>[2x]PRERPHTSGHHGAGEARATAPSTVSPYGPEARAELSSRLTTLRNTLAPATNDPRYLQACGGEKLNRFRDIQCRRQTAVRADLNANYIQVGNTRTIACQYPLQSQLESHFRMLAENRTPVLAVLASSSEIANQRFGMPDYFRQSGTYGSI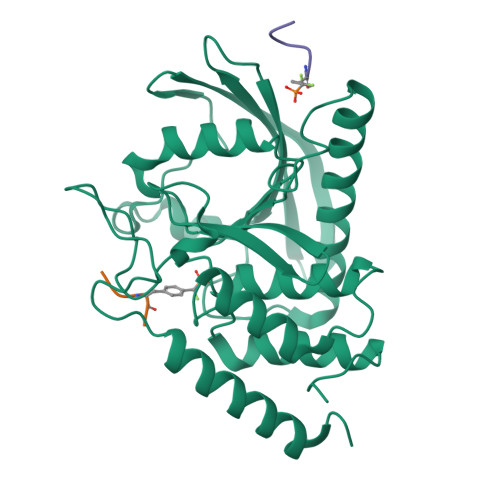TVESKMTQQVGLGDGIMADMYTLTIREAGQKTISVPVVHVGNWPDQTAVSSEVTKALASLVDQTAETKRNMYESKGSSAVADDSKLRPVIHCRAGVGRTAQLIGAMCMNDSRNSQLSVEDMVSQMRVQRNGIMVQKDEQLDVLIKLAEGQGRPLLNS S-(2-{[N-(2-HYDROXY-4-{[HYDROXY(OXIDO)PHOSPHINO]OXY}-3,3-DIMETHYLBUTANOYL)-BETA-ALANYL]AMINO}ETHYL) 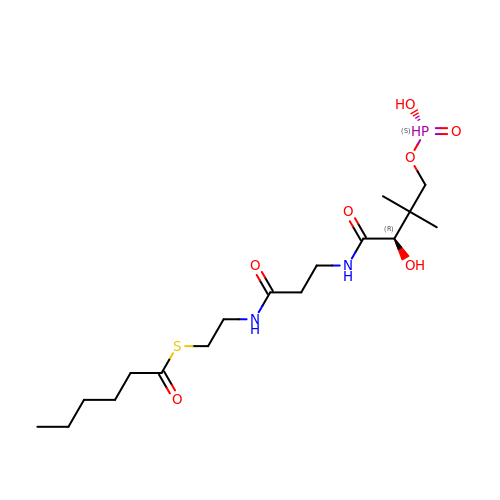HEXANETHIOATE | C17 H33 N2 O7 P S | RXYQLYCKZTXHTF-HNNXBMFYSA-N>MNFDKREERLGTQSVKWDKTGELFGVTDALPMWVADMDFRAPEAITEALKERLDHGIFGYTTPDQKTKDAVCGWMQNRHGWKVNPESITFSPGVVTALSMAVQAFTEPGDQVVVQPPVYTPFYHMVEKNGRHILHNPLLEKDGAYAIDFEDLETKLSDPSVTLFILCNPHNPSGRSWSREDLLKLGELCLEHGVTV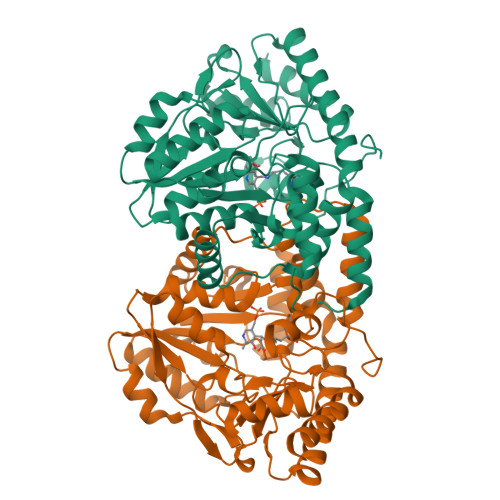VSDEIHSDLMLYGHKHTPFASLSDDFADISVTCAAPSKTFNIAGLQASAIIIPDRLKRAKFSASLQRNGLGGLNAFAVTAIEAAYSKGGPWLDELITYIEKNMNEAEAFLSTELPKVKMMKPDASYLIWLDFSAYGLSDAELQQRMLKKGKVILEPGTKYGPGGEGFMRLNAGCSLATLQDGLRRIKAALS[4x]Cyanobacterial aldehyde-deformylating oxygenase (cADO), which catalyzes the conversion of Cn fatty aldehyde to its corresponding Cn-1 alk(a/e)ne, is a key enzyme in that pathway. Cyanobacterial aldehyde-deformylating oxygenase (cADO) belongs to the superfamily of ferritin-like di-iron proteins and contains a di-iron center. To gain insights into the reaction catalyzed by cADO, we determined structures of wild type ADO from Synechococcus elongates PCC7942 (Se) with different treatment (WT0, no treatment; WT1, co-crystallized with iron; WT-HP, soaked in H2O2), and solved the structures of two SeADO mutants (Y122F and F86YF87Y). SeADO belongs to the di-iron protein family, with conserved sequence of two EX28-29EX2H motifs, in which six conservative amino acids from four helices (Glu32 from helix H1, Glu115 from helix H4, Glu60 & His63 from helix H2, and Glu144 & His147 from helix H5) act as metal ligands.

To explore the effects of H2O2 on ADO activity, a crystal of wild type SeADO was soaked in H2O2, and its structure (WT-HP) was solved. No electron density was visible for the H2O2, probably due to its unstable nature. In our WT-HP structure, a long-chain fatty acid molecule with a bifurcated head-group configuration fits the electron density well. In the WT-HP structure, the helix conformation of H5 was restored, and the two coordinating residues His63 and His147 approach the active site and ligate the Fe1 and Fe2 atoms, respectively. The water molecule that bridges the two iron atoms in the F86YF87Y structure moves towards Fe1 and is not coordinated with Fe2 in the WT-HP structure. The two iron ions are bridged by one carboxylate ligand E60, the Lox ligand and an oxo group. Both iron atoms show saturated coordination with an octahedral geometry. The higher coordination numbers of di-iron center, together with the fact that the crystal was obtained after being treated with strong oxidizer H2O2, lead to the speculation that the WT-HP structure represents an oxidized form of ADO. Furthermore, the coordination mode of two iron atoms in WT-HP structure shows a similar pattern to that observed for the R2 protein of ribonucleotide reductase (RNR-R2), in which the oxo bridge and the coordinated water exist at the di-iron site in the oxidized structure, while both are absent in the reduced structure. We proposed that the Lox ligand is likely to be the analog of the possible intermediate product hemiacetal, thus the WT-HP structure may represent the intermediate state in reaction of cADO, following the entering of dioxygen and its reaction with the substrate.

>[2x]LDFQSESYKDAYSRINAIVIEGEQEAFDNYNRLAEMLPDQRDELHKLAKMEQRHMKGFMACGKNLSVTPDMGFAQKFFERLHENFKAAAAEGKVVTCLLIQSLIIECFAIAAYNIYIPVADAFARKITEGVVRDEYLHRNFGEEWLKANFDASKAELEEANRQNLPLVWLMLNEVADDARELGMERESLVEDFMIAYGEALENIGFTTREIMRMSAYGLAAV>GSLANEKLSQLQKQLEEANDLLRTESDTAVRLRKSHTEMSKSISQLESLNRELQERNRILENSKSQTDKDYYQLQAILEAERRDRGHDSEMIGDLQARITSLQEEVKHLKHNLEKVEGERKEAQDMLNHSEKEKNNLEIDLNYKLKSLQQRLEQEVNEHKVTKARLTD[4x]

Among the downstream targets of activated Rho are two isoforms of Rho-associated kinase (ROCK), ROCK I/ROKβ/p160ROCK and ROCK II/ROKα/Rho kinase, which share 65% sequence identity and 95% sequence similarity at the amino acid level. ROCK is able to regulate the phosphorylation of myosin light chain (MLC) by direct phosphorylation and by inactivation of myosin phosphatase through the phosphorylation of its myosin-binding subunit (MBS). Human ROCK I consists of an N-terminal serine/threonine kinase domain (residues 73–356), a central predicted coiled-coil (residues 422–1102), and a C-terminal pleckstrin homology (PH) domain (residues 1118–1317). Interaction between GTP-Rho and the RBD disrupts ROCK I's autoinhibition and thus activates the kinase.

We obtained crystals of the ROCK coiled-coil domain (ROCK-CC, residues 535–700) in the tetragonal space group P43212. There are four molecules (2 dimers) per asymmetric unit. The structure reveals two long α helices that intertwine to form a two-stranded parallel coiled-coil that is about 220 Å long. ROCK-CC displays 11 consecutive heptad repeats starting at Leu-589 and ending at Lys-666. In the ROCK-CC only about 50% of the a and d positions are taken by hydrophobic residues. Strikingly, near the center of the coiled-coil three consecutive d-a-d positions are occupied by charged residues. These residues (E613, R617 and D620) create an unusual bulge in the coiled-coil. Most interestingly, the charged head group of Arg-617 inserts into the center of the coiled-coil interface and together with Glu-613 and Asp-620, it appears to push apart the two helices. The coiled-coil is bent by about 14° in the region centered around E613/R617/D620, where the inter-helical distance is also at its maximum. How does this autoinhibitory interaction occur if the relevant N- and C-terminal domains are separated by a rod-shaped coiled-coil domain over 220 Å in length? It is tempting to speculate that the E613/R617/D620 irregularity destabilizes the coiled-coil, effectively creating a hinge that allows the coiled-coil to “jackknife”.> SYFSAADVYVPDEWEVAR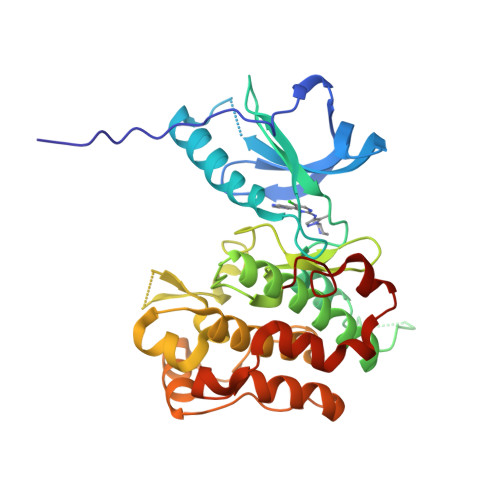EKITMSRELGQGSFGMVYEGVAKGVVKDEPETRVAIKTVNEAASMRERIEFLNEASVMKEFNCHHVVRLLGVVSQGQPTLVIMELMTRGDLKSYLRSLRPEMENNPVLAPPSLSKMIQMAGEIADGMAYLNANKFVHRDLAARNCMVAEDFTVKIGDFGMTRDIYETDYYRKGGKGLLPVRWMSPESLKDGVFTTYSDVWSFGVVLWEIATLAEQPYQGLSNEQVLRFVMEGGLLDKPDNCPDMLFELMRMCWQYNPKMRPSFLEIISSIKEEMEPGFREVSFYYSEENK Rab23 is a member of the Rab family of small GTPases. It plays crucial roles in Hedgehog signaling, ciliary transport, and embryonic development. As a member of the Rab GTPase family, Rab23 acts as a molecular switch by cycling between the GDP-bound inactivated (OFF) state and the GTP-bound activated (ON) state. The structures of the hRab23 in complex with GDP or GMPPNP revealed a typical small GTPase fold of the Ras and Rab family proteins, containing six β-strands and five α-helices.

To elucidate the conformational changes of hRab23 when switching between the ON and OFF state, we determined, by X-ray crystallography, a structure of hRab237-172 (residues 7–172) in complex with GDP, representing the OFF state, and two structures of hRab237-172 in complex with GMPPNP, representing the ON state. The hRab237-172-GMPPNP structures were derived from crystals of different conditions and space groups. In the presence of GMPPNP, the main chain NH of Gly67 in the switch II loop interacts with an O of the γ-phosphate of GMPPNP through a hydrogen bond. This interaction leads to the switch II loop being pulled closer to the GMPPNP ligand, potentially leading to a change in the conformation of switch II, including the loss of a turn in the α2-helix within switch II. Nevertheless, the loops of switch II in both the GMPPNP-bound hRab237-172 structures are still partially disordered (residues 69–73 for the one in space group P31 2 1 and residues 68–73 for the one in space group P2 21 21). The switch I loop adopts a closed conformation in the structure of hRab237-172-GMPPNP (ON state). In both the GMPPNP-bound Rab23 structures, the triphosphate of GMPPNP is fully enclosed by residues from the switch I and P (β1-α1) loops. Residues Tyr38 and Thr41 from switch I differed significantly in terms of their positions in the ON state relative to the OFF state. In the ON state, the side chain hydroxyl of Tyr38 from switch I formed a hydrogen bond with the γ-phosphate of GMPPNP while the side chain of Thr41 chelated Mg2+ trans to the β-phosphate.

> SEVAIKMVVVGNGAVGKSSMIQRYCKGIFTKDYKKTIGVDFLERQIQVNDEDVRLMLWDTAGQEEFDAITKAYYRGAQACVLVFSTTDRESFEAVSSWREKVVAEVGDIPTVLVQNKIDLLDDSCIKNEEAEALAKRLKLRFYRTSVKEDLNVNEVFKYLAEKYLQK> GGSAQPGLVDRYRVTRCRHEVEQGCAVLRATPLADMTPQLLLEVSQGLSRNLKFLTDACALASDKSRDRFSREQFKLGVKCMSTSASALLACVREVKVAPSELARSRCALFSGPLVQAVSALVGF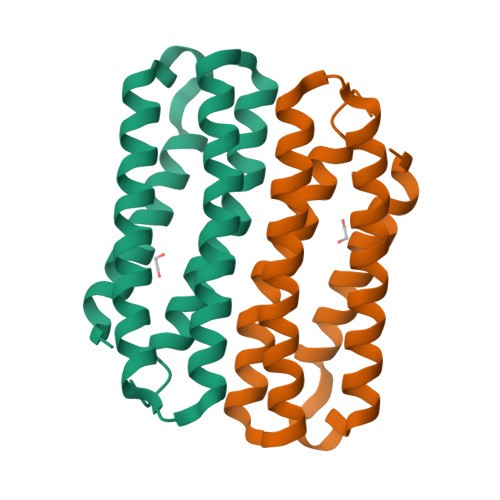ATEPQFLGR>[2x]MGHHHHHHAENLYFQGHMLRLSAPGQLDDDLCLLGDVQVPVFLLRLGEASWALVEGGISRDAELVWADLCRWVADPSQVHYWLITHKHYDHCGLLPYLCPRLPNVQVLASERTCQAWKSESAVRVVERLNRQLLRAEQRLPEACAWDALPVRAVADGEWLELGPRHRLQVIEAHG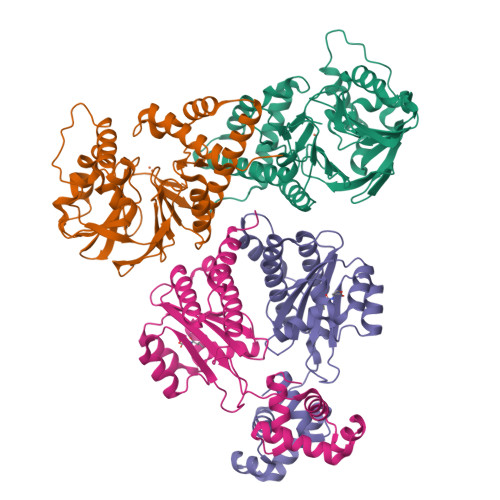HSDDHVVFYDVRRRRLFCGDALGEFDEAEGVWRPLVFDDMEAYLESLERLQRLPTLLQLIPGHGGLLRGRLAADGAESAYTECLRLCRRLLWRQSMGESLDELSEELHRAWGGQSVDFLPGELHLGSMRRMLEILSRQALPLD;>[2x]MRNDGGFLLWWDGLRSEMQPIHDSQGVFAVLEKEVRRLGFDYYAYGVRHTIPFTRPKTEVHGTYPKAWLERYQMQNYGAVDPAILNGLRSSEMVVWSDSLFDQSRMLWNEARDWGLCVGATLPIRAPNNLLSVLSVARDQQNISSFEREEIRLRLRCMIELLTQKLTDLEHPMLMSNPVCLSHREREILQWTADGKSSGEIAIILSISESTVNFHHKNIQKKFDAPNKTLAAAYAAALGLI> CASSSSGDRPQGR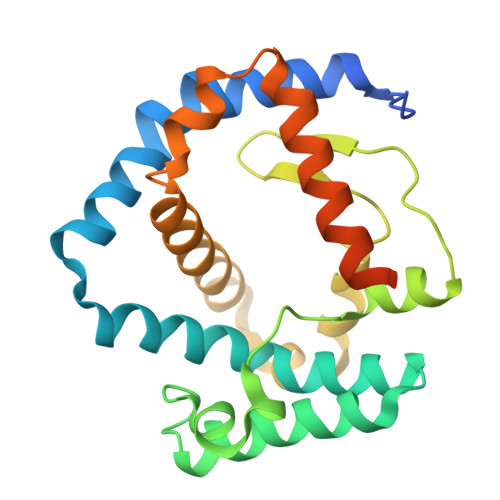SDPLEGFNRTMFNFNFNVVDPYVLRPVAVAWRDYVPQPARNGLSNFTSNLEEPAVMVNYFLQGDPYKGMVHFTRFFLNTILGMGGLIDVAGMANPQLQRVEPHRFGSTLGHYGVGYGPYVQLPFYGSFTLRDEGGDMADGLYPVLSWLTWPMSIGKWAVEGIETRAQLLDSDGLLRQSSDPYILMREAYFQRHDFIANGGKLTPADNPNAQAIQDELKDIDSQ>MKHTELRAAVLDALEKHDTGATFFDGRPAVFDEADFPAVAVYLTGAEYTGEELDSDTWQAELHIEVFLPAQVPDSELDAWMESRIYPVMSDIPALSDLITSMVASGYDYRRDDDAGLWSSADLTYVITYEM[6x];>[6x]MPVPNPTMPVKGAGTTLWVYKGSGDPYANPLSDVDWSRLAKVKDLTPGELTAESYDDSYLDDEDADWTATGQGQKSAGDTSFTLAWMPGEQGQQALLAWFNEGDTRAYKIRFPNGTVDVFRGWVSSIGKA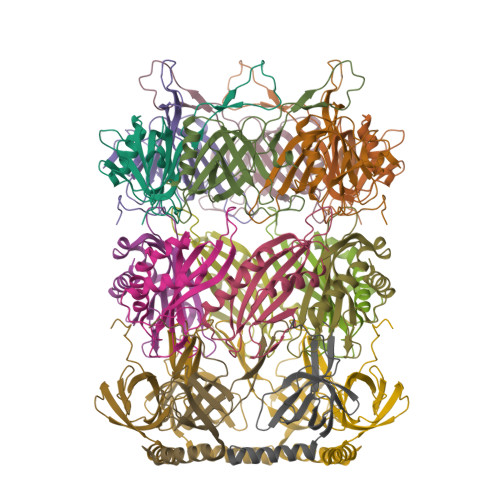VTAKEVITRTVKVTNVGRPSMAEDRSTVTAATGMTVTPASTSVVKGQSTTLTVAFQPEGVTDKSFRAVSADKTKATVSVSGMTITVNGVAAGKVNIPVVSGNGEFAAVAEITVTAS;>MADFDNLFDAAIARADETIRGYMGTSATITSGEQSGAVIRGVFDDPENISYAGQGVRVEGSSPSLFVRTDEVRQLRRGDTLTIGEENFWVDRVSPDDGGSCHLWLGRGVPPAVNRRR[6x]>[4x]AETVSFNFNSFSEGNPAINFQGDVTVLSNGNIQLTNLNKVNSVGRVLYAMPVRIWSSATGNVASFLTSFSFEMKDIKDYDPADGIIFFIAPEDTQIPAGSIGGGTLGVSDTKGAGHFV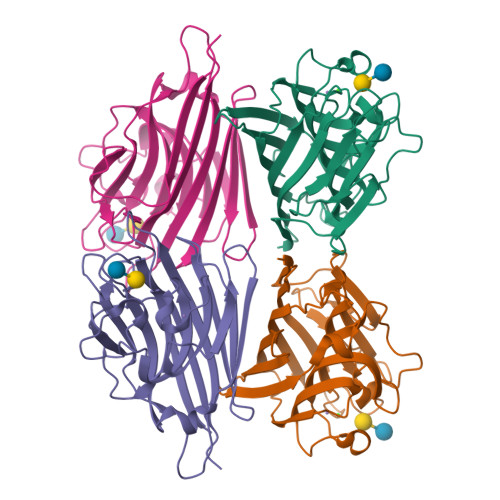GVEFDTYSNSEYNDPPTDHVGIDVNSVDSVKTVPWNSVSGAVVKVTVIYDSSTKTLSVAVTNDNGDITTIAQVVDLKAKLPERVKFGFSASGSLGGRQIHLIRSWSFTSTLITT>MEIVEYPDPILRAKNKRIDIFDENLKNLVDAMFDVMYKTDMIGLSAPQVGLNVQLMVFNPAGEPGEGKEIVLVNPKIKKYSDKLVPFDEGCLSFPGIYAEVVRPQSVKIDARDITGERFSISLSRLPARIFQHEYDHLEGVL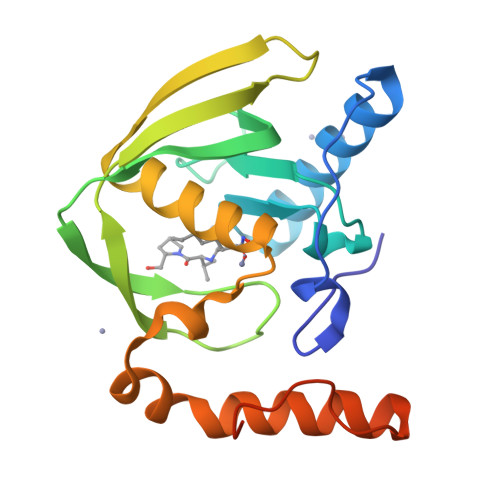FFDRMTDQVLDSIREELEALEKKYEEKTGLPSPERVEARQKRKAGVGFGKR[4x]fipronil | 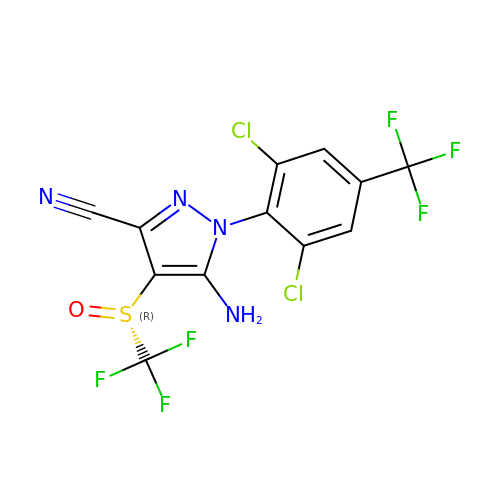C12 H4 Cl2 F6 N4 O S | ZOCSXAVNDGMNBV-AREMUKBSSA-N> TLKLCSPEEFTRLCREKTQEIYPIKEANGRTRKALIICNTEFKHLSLRYGANFDIIGMKGLLEDLGYDVVVKEELTAEGMESEMKDFAALS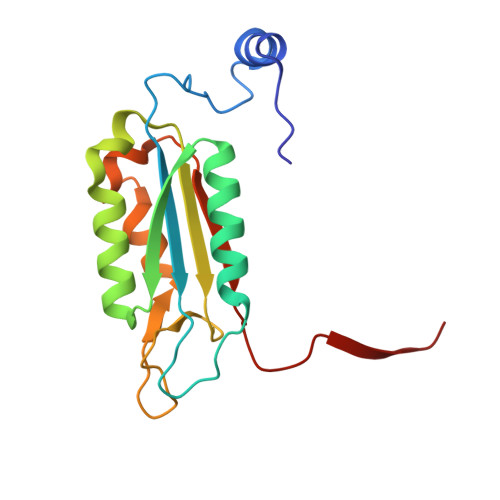EHQTSDSTFLVLMSHGTLHGICGTMHSEKTPDVLQYDTIYQIFNNCHCPGLRDKPKVIIVQAARGGNSGEMWIRE>GSQIPASEQETLVRPKPLLLKLLKSVGAQKDTYTMKEVLFYLGQYIMTKRLYDEKQQHIVYCSNDLLGDLFGVPSFSVKEHRKIYTMIYRNLVVVN[3x];>[3x]FSDXSSVP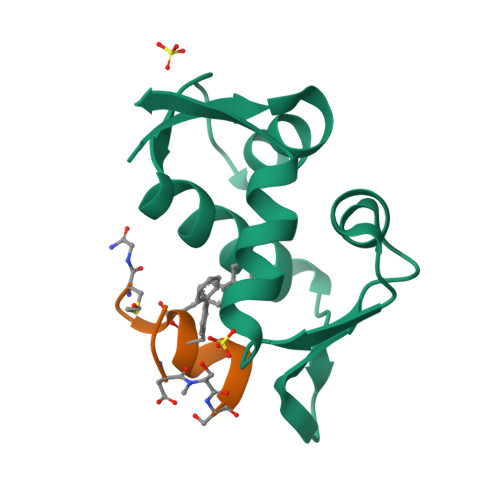NFFRNCX>[2x]MSHVEYSRITKFFQEQPLEGYTLFSHRSAPNGFKVAIVLSELGFHYNTIFLDFNLGEHRAPEFVSVNPNARVPALIDHGMDNLSIWESGAILLHLVNKY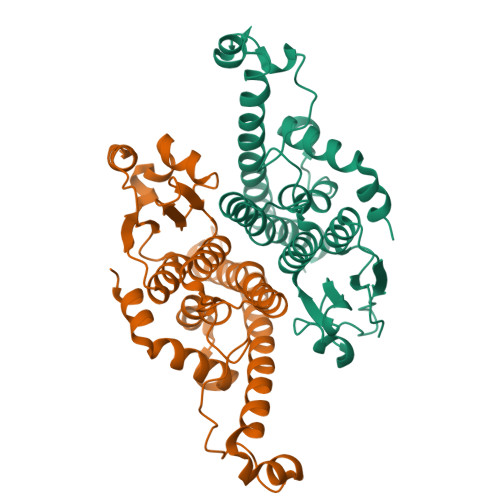YKETGNPLLWSDDLADQSQINAWLFFQTSGHAPMIGQALHFRYFHSQKIASAVERYTDEVRRVYGVVEMALAERREALVMELDTENAAAYSAGTTPMSQSRFFDYPVWLVGDKLTIADLAFVPWNNVVDRIGINIKIEFPEVYKWTKHMMRRPAVIKALRGE>[2x]GPEFMSAIKP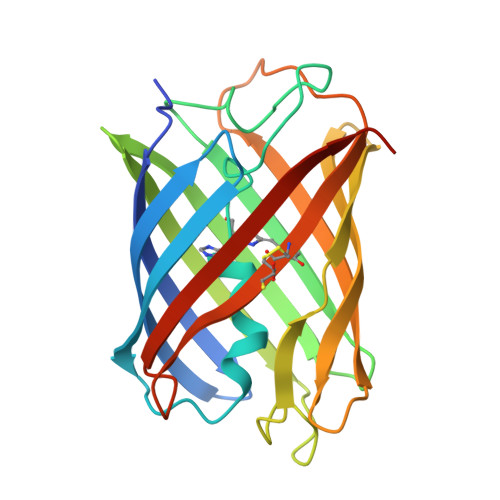DMKIKLRMEGNVNGHHFVIDGEGTGKPFEGKQSMDLEVKEGGPLPFAFDILTTAFHYGNRVFAKYPDNIQDYFKQSFPKGYSWERSMTFEDGGICNARNDITMEGDTFYNKVRFYGTNFPANGPVMQKKTLKWEPSTEKMYVRDGVLTGDIEMALLLEGGAHYRCDFRTTYKAKEKGVKLPGAHFVDHCIEILSHDKDYNKVKLYEHAVAHSGLPDNARR NExo is an enzyme from Neisseria meningitidis that is specialized in the removal of the 3′-phosphate and other 3′-lesions, which are potential blocks for DNA repair. NExo is a highly active DNA 3′-phosphatase, and although it is from the class II AP family it lacks AP endonuclease activity. NExo folds into two planes of beta sheets sandwiched between two planes of alpha helices. Notably, the amino acids residues of the active site of the NExo 3′-phosphatase are identical to the active sites of NApe, E. coli Exo III and human APEX1.

In addition, a catalytic point mutant (D146N) was used to obtain the structures of both the substrate and product DNA complexes in the presence of Mg2+, the essential metal ion cofactor. The NExo mutation D146N is analogous to the D210N mutation which inactivates human APEX1 (37–39), and our biochemical analysis demonstrates that D146N completely abolishes activity in NExo. The position of divalent metal ion cofactors was determined for the inactive D146N in complex with substrate DNA and Mg2+, and for the product DNA complex with Mn2+. In the D146N structure with the 3′-phosphate substrate, we see that the scissile phosphoester bond that links the 3′-oxygen (O1P) to the phosphate is bound within the active site of NExo, and is oriented towards the mutated catalytic residue D146N. Recognition of the 3′-phosphate is mediated via hydrogen bonds between the 3′-phosphate and neighbouring residues N148, H247, N7 and Y105. The substrate bound structure of NExo has a Mg2+ ion coordinated between the well-conserved D146, N7, N9 and E34, which are positioned on the leaving group side of the scissile phosphate bond. Therefore, the Mg2+ ion is well positioned to stabilize the increased negative charge of the pentavalent transition state and the displacement of negative charge onto the 3′-oxygen during the dissociative phase of the reaction. That the D146N mutation completely abolishes activity of the enzyme indicates a critical role for this residue in catalysis. Catalytic residue D146 is positioned for an in-line attack of the phosphate centre for direct coordination and deprotonation of the attacking water.

> GAMKITTWNVNSLNVRLPQVQNLLADNPPDILVLQELKLDQDKFPAAALQMMGWHCVWSGQKTYNGVAIVSRSVPQDVHFGLPALPDDPQRRVIAATVSGVRVINVYCVNGEALDSPKFKYKEQWFAALTEFVRDEMTRHGKLVLLGNFNIAPADADCYDPEKWHEKIHCSSVERQWFQNLLDLGLTDSLRQVHPEGAFYTWFDYRGAMFQRKLGLRIDHILVSPAMAAALKDVRVDLETRALERPSDHAPVTAEFDW> MKLKQIASALMMLGISPLAFADFTIQDIRVEGLQRTEPSTVFNYLPVKVGDTYNDTHGSAIIKSLYATGFFDDVRVETADGQLLLTVIERPTIGSLNITGAKMLQNDAIKKNLESFGLAQSQYFNQATLNQAVAGLKEEYLGRGKLNIQITPKVTKLARNRVDIDITIDEGKSAKITDIEFEGNQVYSDRKLMRQMSLTEGGIWTWLTRSDRFDRQKFAQDMEKVTDFYQNNGYFDFRILDTDIQTNEDKTRQTIKITVHEGGRFRWGKVSIEGDTNEVPKAELEKLLTMKPGKWYERQQMTAVLGEIQNRMGSAGYAYSEISVQPLPNAGTKTVDFVLHIEPGRKIYVNEIHITGNNKTR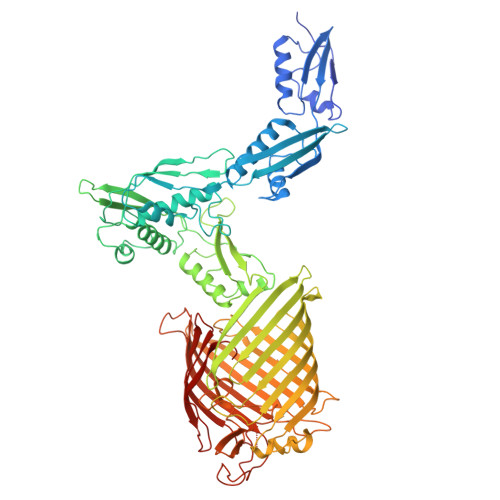DEVVRRELRQMESAPYDTSKLQRSKERVELLGYFDNVQFDAVPLAGTPDKVDLNMSLTERSTGSLDLSAGWVQDTGLVMSAGVSQDNLFGTGKSAALRASRSKTTLNGSLSFTDPYFTADGVSLGYDIYGKAFDPRKASTSVKQYKTTTAGGGVRMGIPVTEYDRVNFGLAAEHLTVNTYNKAPKRYADFIRKYGKTDGADGSFKGLLYKGTVGWGRNKTDSASWPTRGYLTGVNAEIALPGSKLQYYSATHNQTWFFPLSKTFTLMLGGEVGIAGGYGRTKEIPFFENFYGGGLGSVRGYESGTLGPKVYDEYGEKISYGGNKKANVSAELLFPMPGAKDARTVRLSLFADAGSVWDGRTYTAAENGNNKSVYSENAHKSTFTNELRYSAGGAVTWLSPLGPMKFSYAYPLKKKPEDEIQRFQFQLGTTF>MKVVKEFSVCGGRLIKLSHNSNSTKTSMNVNIYLPKHYYAQDFPRNKRIPTVFYLSGLTCTPDNASEKAFWQFQADKYGFAIVFPDTSPRGDEVANDPEGSWDFGQGAGFYLNATQEPYAQHYQMYDYIHKELPQTLDSHFNKNGDVKLDFLDNVAITGHSMGGYGAICGYLKGYSGKRYKSCSAFAPIVNPSNVPIGQKAFKGYLGEEKAQW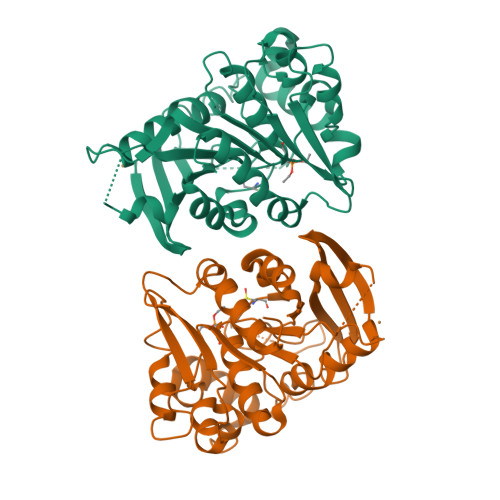EAYDPCLLIKNIRHVGDDRILIHVGDSDPFLEEHLKPELLLEAVKATSWQDYVEIKKVHGFDHSYYFVSTFVPEHAEFHARNLGLI[2x]> GSPSTCTVTIEVLGHELDFAQDPNSKHLGTTVWDASMVFAKYLGKNSRKGRFSSSKLKGKRAIELGAGCGVAGFALAMLGCDVVTTDQKEVLPLLKRNVEWNTSRIVQMNPGSAFGSLRVAELDWGNEDHITAVEPPFDYVIGTDVVYSEQLLEPLLRTILALSGPKTTVMLGYEIRSTVVHEKMLQMWKDNFEVKTIPRSKMDGEYQDPSIHLYIMAQKSAAESSAAA

pmcp97, also known as CDC48 or valosin-containing protein (VCP), is a hexameric, ring-shaped AAA+ ATPase (ATPase associated with diverse cellular activities) that can extract ubiquitinated and nonubiquitinated substrate proteins from protein complexes and membranes. ASPL (alveolar soft-part sarcoma locus; also known as UBXD9, TUG, or ASPSCR1) is a unique p97 adaptor protein that regulates p97 activity by disassembling the p97 hexamer into smaller oligomers. One example is trimethylation of p97 at residue Lys315, a modification introduced by METTL21D (also known as VCP-KMT or NVM-1). Here, we report the crystal structures of a human p97:ASPL:METTL21D heterotrimeric complex and of the plant methyltransferase AtMETTL21D.

To our surprise, AtMETTL21D was unable to trimethylate AtCDC48. Since the AtCDC48:PUX1:AtMETTL21D complex did not crystallize, we analyzed the structure of AtMETTL21D to gain insight into its mode of action. The crystal structure showed AtMETTL21D in a premethylation state and crystal packing of AtMETTL21D suggested an automethylation mode with residue Lys56 from one molecule pointing toward the active site of the neighboring molecule. First, it revealed that the lysine residue pointing to the binding pocket was indeed not trimethylated. However, when we probed our AtCDC48 samples with an anti-monomethyl-lysine antibody, we observed that AtMETTL21D monomethylated itself, as well as AtCDC48 in the presence of PUX1. Secondly, the structure revealed a difference in the hydrophobic cage that accommodates the methylated ε-amino group. Instead of a Val-Trp-Tyr cage, the plant enzyme contains a Leu-Trp-Tyr cage. We hypothesized that substitution of valine by the larger leucine residue introduces steric hindrance on the possible methylation level. Subsequently, substitution of leucine with valine in plant AtMETTL21D resulted in gain of trimethylation activity. Therefore, we suggest that the leucine to valine substitution in the hydrophobic cage of A. thaliana METTL21D acts as a switch that shifts the methyltransferase activity from monomethylation to trimethylation.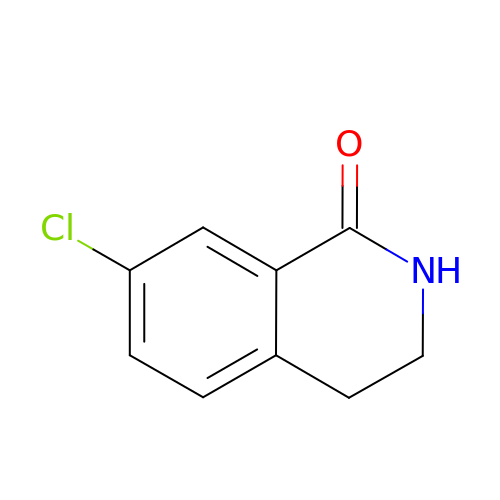7-chloro-3,4-dihydroisoquinolin-1(2H)-one | C9 H8 Cl N O | NMZRTRAYSHQMPR-UHFFFAOYSA-N>[2x]MEFTVSTTEDLQRYRTECVSSLNIPADYVEKFKKWEFPEDDTTMCYIKCVFNKMQLFDDTEGPLVDNLVHQLAHGRDAE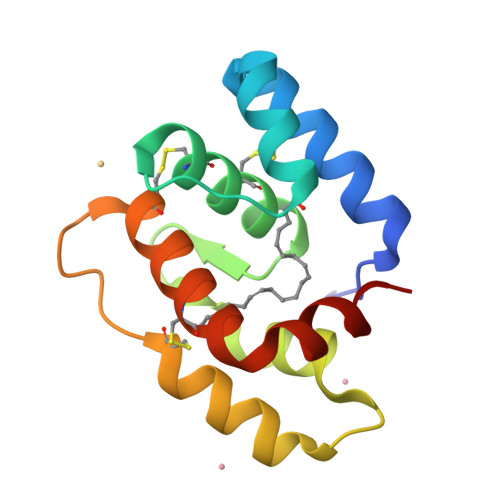EVRTEVLKCVDKNTDNNACHWAFRGFKCFQKNNLSLIKASIKKD> ATATAAPSELDDVGVSAAAESIIQYAINFARASETYEVHSWMVLMGILKYETCTAAKILKSLGL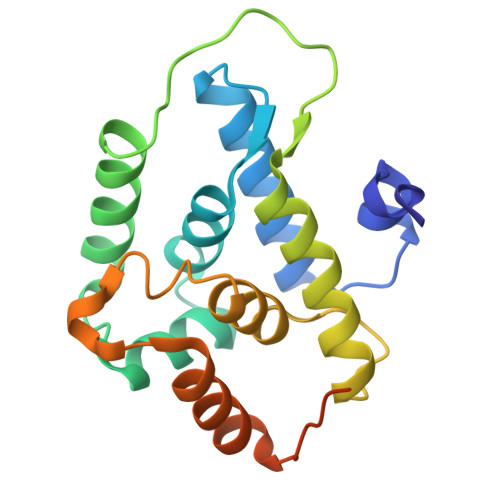EDLYGAWNEVLWALNVCDGLQPRSFVTDIKFADRAFKVITAASDFAVWHGKDKMYSEDVLMALAAGGVLEDLFPDLNLSFERVRKAVEKESGRRYQLPDETEEAGPLKSEDDVSFL> AMPFEIEVLLPGELSPAETSALQKCEGKIITFSTLRHRASLVDIALSSYYING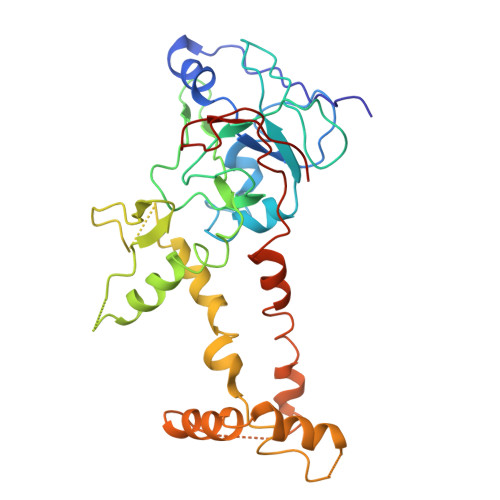APPDTLSLLEAYRMRFAAVITRVIPGKLLAHAIGVGTPTPGLFIQNTSPVDLCNGDYICLLPPVFGSADSIRLDSVGLEIVFPLTIPQTLMREIIAKVVARAVEDLNPDPDLNVLYYNGARLSLVADVQQLASDAAIRTLVLNLMFSINEGCLLILALIPRLLALGYVNALLQMQSVTREAAQLIHPEAPMLMRRLPIYETISSWISTSSRLGDTLGTRAILRVCVFDGPSTVHPGDRTAVIQV> GLPVMNTPGSNQYLTADNFQSPCALPEFDVTPPIDIPGEVKNMMELAEIDTMIPFDLSATKKNTMEMYRVRLSDKPHTDDPILCLSLSPASDPRLSHTMLGEILNYYTHWAGSLKFTFMFCGSMMATGKLLVSYAPPGADPPKK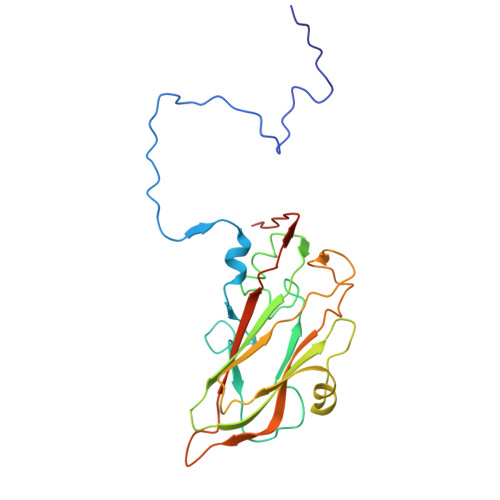RKEAMLGTHVIWDIGLQSSCTMVVPWISNTTYRLTIDDSFTEGGYISVFYQTRIVVPLSTPREMDILGFVSACNDFSVRLLRDTTHIEQKALAQ>[2x]MHHHHHHLVPRGSPARIGYYEIDRTIGKGNFAVVKRATHLVTKAKVAIKIIDKTQLDEENLKKIFREVQIMKMLCHPHIIRLYQVMETERMIYLVTEYASGGEIFDHLVAHGRMAEKEARRKFKQIVTAVYFCHCRNIVHRDLKAENLLLDANLNIKIADFGFSNLFTPGQLLKDWCGSPPYAAPELFEGKEYDGPKVDIWSLGVVLYVLVCGALPFDGSTLQNLRARVLSGKFRIPFFMSTECEHLIRHMLVLDPNKRLSMEQICKHKWMKLGDADPNFDRLIAECQQLKEERQVDPLNEDVLLAMEDMGLDKEQTLQSLRSDAYDHYSAIYSLLCDRHKRHKTLRL

The salt-inducible kinase (SIK) family comprises three isoforms (SIK1, SIK2, and SIK3) that belong to the AMP-activated protein kinase (AMPK) family of serine/threonine protein kinases. SIKs have been implicated in the regulation of several physiological processes, including circadian rhythms, bone formation, skin pigmentation, metabolism, and modulation of inflammatory cytokine production. The SIKs control gene regulation and act as a molecular switch, and inhibition has been shown to reprogram myeloid cell types to an immunoregulatory phenotype. Inhibition of SIKs in stimulated innate immune cells and mouse models has been associated with a dual mechanism of action consisting of a reduction of pro-inflammatory cytokines and an increase of immunoregulatory cytokine production, suggesting a therapeutic potential for inflammatory diseases.

The crystal structure of SIK3 (60-394 T221D) in a complex with 22 was determined to 3.1 Å. The structure contains a classical bilobed kinase catalytic domain with a flexible hinge region connecting the two lobes and forming a hydrophobic cleft serving as the binding site for ATP where compound 22 is bound. In the crystal structure, the kinase domain of SIK3 adopts an active-like conformation (DFG-in, αC-helix-in). The kinase catalytic domain is connected by a linker to an α-helical ubiquitin-associated (UBA) domain. The UBA domain packs onto the N-terminal lobe of the catalytic domain, forming an extensive interface consisting of 536 Å2 in buried surface area, distal to the catalytic cleft where 22 is located. Compound 22 binds in the ATP site with the protein adopting an active-like conformation (DFG-in, αC-helix-in) and as such can be classed as a type 1 kinase inhibitor. The benzimidazole nitrogen of 22 establishes a hydrogen bond interaction with the backbone NH of Ala145 at the hinge. The phenyl ring is out of plane relative to the benzimidazole scaffold, and the side chains of Val80 and Ala205 provide lipophilic contacts to the substituted phenyl group. The amide group forms a hydrogen bond contact with Lys95 but not with Asp206. The pyrazole ring is coplanar with the benzimidazole scaffold, allowing a displaced π–π interaction with Tyr144 and a weak hydrogen bond between the slightly polarized C–H group of the pyrazole and the carbonyl moiety of Ala145.>[6x]MGSIGSMGKPIEGFLVAAIQFPVPIVNSRKDID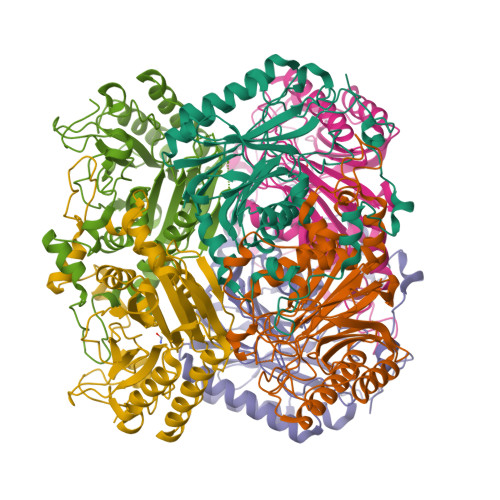HNIESIIRTLHATKAGYPGVELIIFPEYSTQGLNTAKWLSEEFLLDVPGKETELYAKACKEAKVYGVFSIMERNPDSNKNPYNTAIIIDPQGEIILKYRKLFPWNPIEPWYPGDLGMPVCEGPGGSKLAVCISHDGMIPELAREAAYKGCNVYIRISGYSTQVNDQWILTNRSNAWHNLMYTVSVNLAGYDNVFYYFGEGQICNFDGTTLVQGHRNPWEIVTGEIYPKMADNARLSWGLENNIYNLGHRGYVAKPGGEHDAGLTYIKDLAAGKYKLPWEDHMKIKDGSIYGYPTTGGRFGK>[2x]GMTNHNNSGKKKVAILIEQAVEDTEFIIPCNGLKQAGFEVVVLGSRMNEKYKGKRGRLSTQADGTTTEAIASEFDAVVIPGGMAPDKMRRNPNTVRFVQEAMEQGKLVAAVCHGPQVLIEGDLLRGKQATGFIAISKDMMNAGADYLDEALVVDGN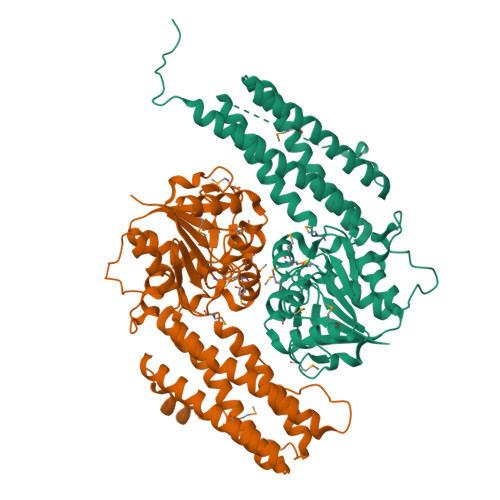LITSREPGDLAIFTTAILSRLGYGGKDAALPDEKDRNAEWWKLADAWGGSTKGDIVRGLNTALGGERYSLEALEKYTEKESDVEAKALFQEMITNKQRHIEYLETYLTRLGEKPSLSANIANQYAKVKTALTGSDDIYQIRSALGDIQTGIGDIGNLCAMYTDPIATAIFKEIYKDLVKYEQRLVSLYRTRTNATVQPPKPTTGAAVSM>[4x]VGAFRSGLEDKVSKQLESKGIKFEYEEWKVPYVIPASNHTYTPDFLLPNGIFVETKGLWESDDRKKHLLIREQHPELDIRIVFSSSRTKLYKGSP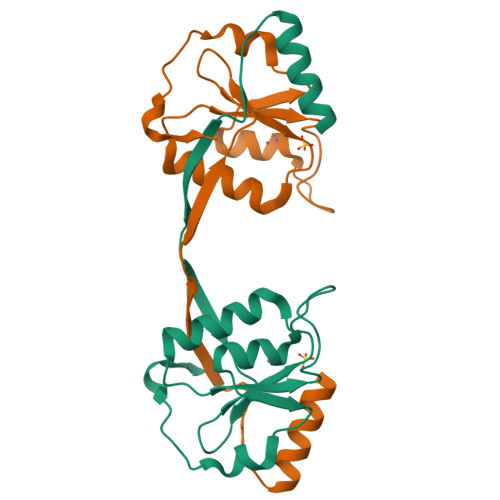TSYGEFCEKHGIKFADKLIPAEWIKEPKKEVPFDRLKRKGGKK> DEMFSDIYKIREIAD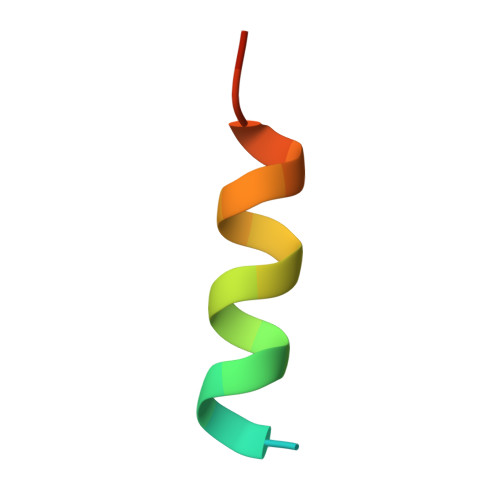GLCLEV> MELTPREKDKLLLFTAALVAERRLARGLKLNYPESVALISAFIMEGARDGKSVASLMEEGRHVLTREQVMEGVPEMIPDIQVEATFPDGSKLVTVHNPII;> MIPGEYHVKPGQIALNTGRATCRVVVENHGDRPIQVGSHYHFAEVNPALKFDRQQAAGYRLNIPAGTAVRFEPGQKREVELVAFAGHRAVFGFRGEVMGPL;> SNISRQAYADMFGPTVGDKVRLADTELWIEVEDDLTTYGEEVKFGGGKVIRDGMGQGQMLAADCVDLVLTNALIVDHWGIVKADIGVKDGRIFAIGKAGNPDIQPNVTIPIGAATEVIAAEGKIVTAGGIDTHIHWICPQQAEEALVSGVTTMVGGGTGPAAGTHATTCTPGPWYISRMLQAADSLPVNIGLLGKGNVSQPDALREQVAAGVIGLAIHEDWGATPAAIDCALTVADEMDIQVALHSDTLNESGFVEDTLAAIGGRTIHTFHTEGAGGGHAPDIITACAHPNILPSSTNPTLPYTLNTIDEHLDMLMVCHHLDPDIAEDVAFAESRIRRETIAAEDVLHDLGAFSLTSSDSQAMGRVGEVILRTWQV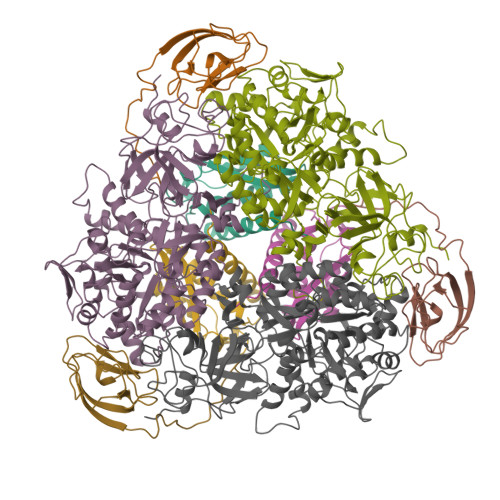AHRMKVQRGALAEETGDNDNFRVKRYIAKYTINPALTHGIAHEVGSIEVGKLADLVVWSPAFFGVKPATVIKGGMIAIAPMGDINASIPTPQPVHYRPMFGALGSARHHCRLTFLSQAAAANGVAERLNLRSAIAVVKGCRTVQKADMVHNSLQPNITVDAQTYEVRVDGELITSEPADVLPMAQRYFLF(3R)-3-(2,4-dichlorophenyl)-N~1~-hydroxy-N~5~-pentylpentanediamide | C16 H22 Cl2 N2 O3 | 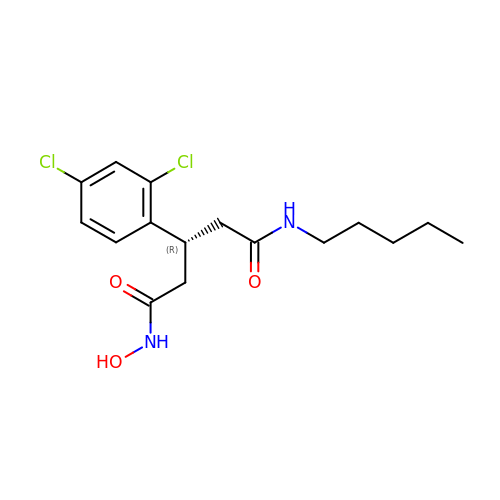FHIDAHOTTVOIDA-LLVKDONJSA-N(1R,3S)-5-methyl-2-[(1S)-2-naphthalen-1-yloxy-1-oxidanyl-ethyl]cyclohexane-1,3-diol 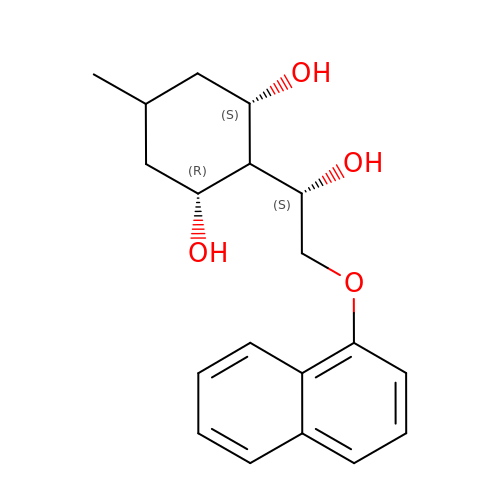| C19 H24 O4 | LTDHFDASOVNXLA-ZJADBGPTSA-N>MTKENICIVFGGKSAEHEVSILTAQNVLNAIDKDKYHVDIIYITNDGDWRKQNNITAEIKSTDELHLENGEALEISQLLKESSSGQPYDAVFPLLHGPNGEDGTIQGLFEVLDVPYVGNGVLSAASSMDKLVMKQLFEHRGLPQLPYISFLRSEYEKYEHNILKLVNDKLNYPVFVKPANLGSSVGISKCNNEAELKEGIKEAFQFDRKLVIEQGVNAREIEVAVLGNDYPEATWPGEVVKDVAFYDYKSKYKDGKVQLQIPADLDEDVQLTLRNMALEAFKATDCSGLVRADFFVTEDNQIYINETNAMPGFTAFSMYPKLWENMGLSYPELITKLIELAKERHQDKQKNKYKID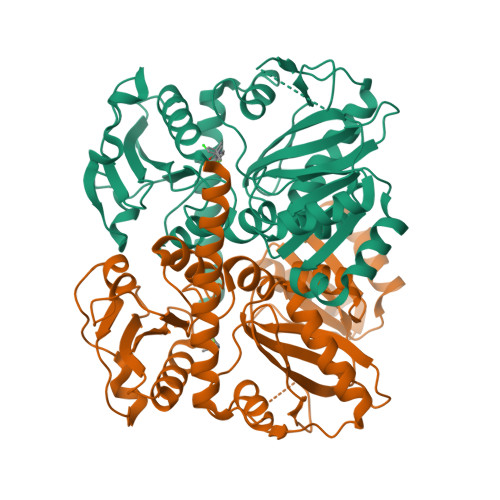RSHH[2x]> EMATVKTTHRTIAGWDGTPLGAFVIEPQDAGGGRYPLLVMPSSWAVPSVEYVGVAQSLAQRGYVVISYSSRGFWESGGSIDIAGPSTVEDV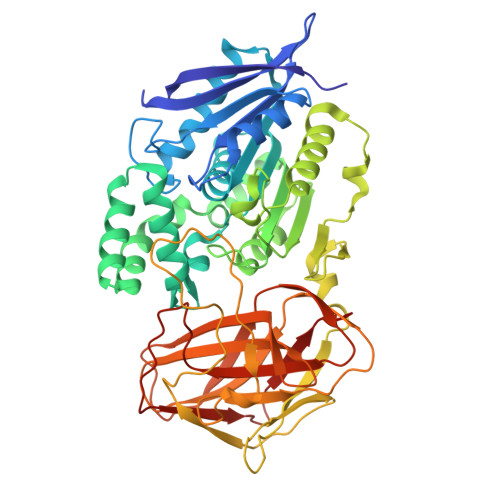SALIDWALDNTRADPDRIGVSGISYGAGTSLLAAARDPRIKAVAALSGWADLQASLYSNDTPSAQGIALLVAAGLVTGRPGAELATINRNVLAGNYQGAVDSLLPVAAQRSPAASIDEINANQPAVFLANAFNDSLFPPGQLVDFFNRLKGPKQLQMRHGDHALNEALGALGIPNEVYDQVGDWFDHYLKAVANGIDRQPAVQLKSQKGSWSSYPDWQATSKGAVSYGLTAPSGLLLPTGGLAEHGGGTGWNYRIGSGLLTAANSGVAMASGALQMINLPPGAYVPFVGRSAAGVWQGPIQWSAKRLDGAPEVRLTVTPSRANTTLYAYLYAEDVLGNGQLISHKPYTLRGATPGQAKTLDLRLEASSWNLPAGSRLTLVVDTVDLRYAGISQLGGAVTFTSPANAPSVLKVPLH> DPCSVTEYSGLATAVSSCKNIVLNGFQVPTGKQLDLSSLQNDSTVTFKGTTTFATTADNDFNPIVISGSNITITGASGHVIDGNGQAYWDGKGSNSNSNQKPDHFIVVQKTTGNSKITNLNIQNWPVHCFDITGSSQLTISGLILDNRAGDKPNAKSGSLPAAHNTDGFDISSSDHVTLDNNHVYNQDDCVAVTSGTNIVVSNMYCSGGHGLSIGSVGGKSDNVVDGVQFLSSQVVNSQNGCRIKSNSGATGTIN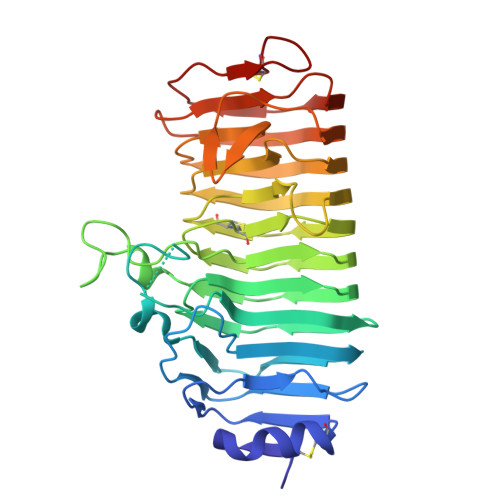NVTYQNIALTNISTYGVDVQQDYLNGGPTGKPTNGVKISNIKFIKVTGTVASSAQDWFILCGDGSCSGFTFSGNAITGGGKTSSCNYPTNTCPS> KKLIPILEKIPEVELPVKEITFKEKLKWTGIVLVLYFIMGCIDVYTAGAQIPAIFEFWQTITASRIGTLITLGIGPIVTAGIIMQLLVGSGIIQMDLSIPE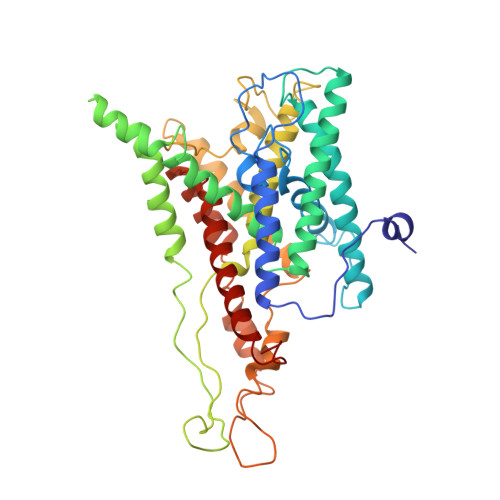NRALFQGCQKLLSIIMCFVEAVLFVGAGAFGILTPLLAFLVIIQIAFGSIILIYLDEIVSKYGIGSGIGLFIAAGVSQTIFVGALGPEGYLWKFLNSLIQGVPNIEYIAPIIGTIIVFLMVVYAECMRRRIVVNYAKRQQGRRVYAAQSTHLPLKVVYVSNIPVILAAALFANIQLWGLALYRMGIPILGHYEGGRAVDGIAYYLSTPYGLSSVISDPIHAIVYMIAMIITCVMFGIFWVETTGLDPKSMAKRIKKSGAFVPGIRPGEQTAKYIEHRLKRYIPPLTVMSSAFVGFLATIANFIGALGGGTGVLLTVSIVYRMYEQLLREKVSELHPAIAKL>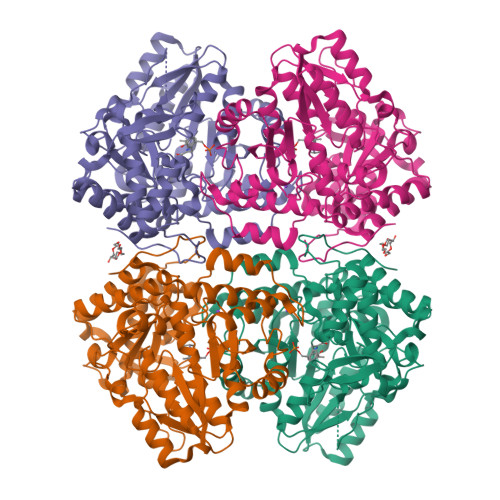[2x]MNYPAEPFRIKSVETVSMIPRDERLKKMQEAGYNTFLLNSKDIYIDLLTDSGTNAMSDKQWAGMMMGDEAYAGSENFYHLERTVQELFGFKHIVPTHQGRGAENLLSQLAIKPGQYVAGNMYFTTTRYHQEKNGAVFVDIVRDEAHDAGLNIAFKGDIDLKKLQKLIDEKGAENIAYICLAVTVNLAGGQPVSMANMRAVRELTAAHGIKVFYDATRCVENAYFIKEQEQGFENKSIAEIVHEMFSYADGCTMSGKKDCLVNIGGFLCMNDDEMFSSAKELVVVYEGMPSYGGLAGRDMEAMAIGLREAMQYEYIEHRVKQVRYLGDKLKAAGVPIVEPVGGHAVFLDARRFCEHLTQDEFPAQSLAASIYVETGVRSMERGIISAGRNNVTGEHHRPKLETVRLTIPRRVYTYAHMDVVADGIIKLYQHKEDIRGLKFIYEPKQLRAFTARFDYI> MSQSNRELVVDFLSYKLSQKGYSWSQPMAAVKQALREAGDEFELRYRRAFSDLTSQLHITPGTAYQSFEQVVNELFRDGVNWGRIVAFFSFGGALCVESVDKEMQVLVSRIASWMA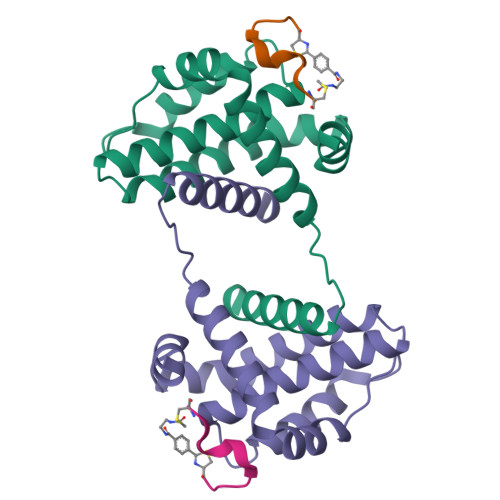TYLNDHLEPWIQENGGWDTFVDLYG;> APIRYEWDEFC>[6x]MSCKKRDDYLEWPEYFMAVAFLSAQRSKDPNSQVGACIVNSENKIVGIGYNGMPNGCSDDVLPWRRTAENKLDTKYPYVCHAELNAIMNKNLTDVKGCSMYVALF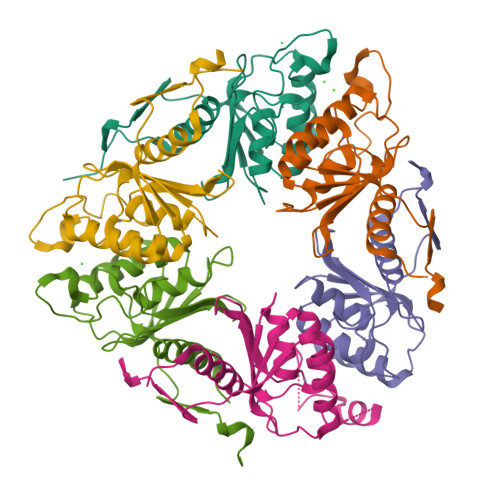PCNECAKLIIQAGIKEVIFMSDKYHDSDEATAARLLFNMAGVTFRKFIPKCSKIVIDFDSINSRPSAHHHHHH>[6x]GSGEGVQPQEYIGIKLELINYTTLLEEQREQQQEGEEEGDGMDDSLAEKLNIKLPRFYSNPKNKAIFDQLWENQVDNAKVYLLAATLRPETMVGQTNCWVLPTGRYGAYYINKDEVIIVSEHAAVNMAHQGLNNNKPFGELDFISEISGSDL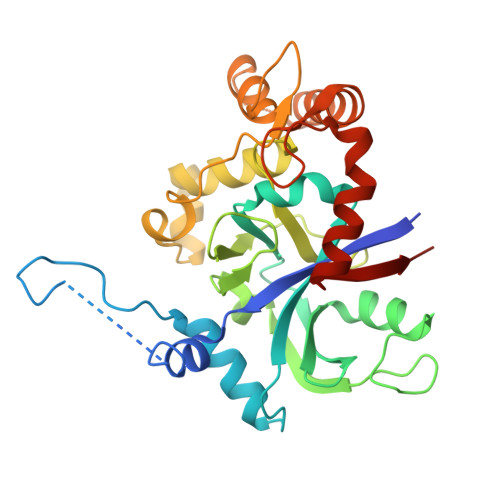LLATVRAPLSPYEQIFVLPLETIKMDKGTGIVTSVPSDAPDDYACYKDILENRNGIAEKYGVDVGLMLEPYSPLPIIEIPDIGTLSAVRLCEESNVSSLHDRAKLTQIKEICYTKGFYTGIMKMGPFAGQSVKDCKQSCRDLLVQNNQCIVYSEPESEV> AQVINTFDGVADYLQTYHKLPDNYITKSEAQALGWVASKGNLADVAPGKSIGGDIFSNREGKLP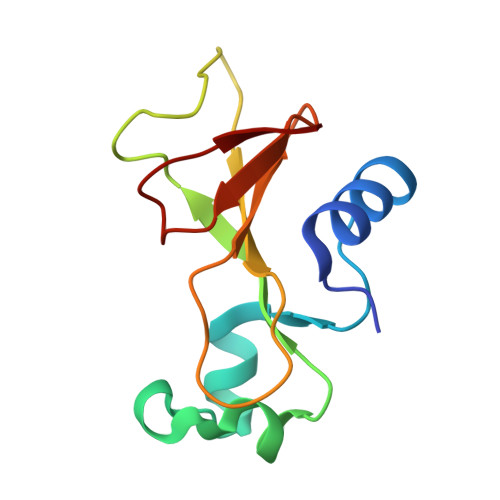GKSGRTWREADINYTSGFRNSDRILYSSDWLIYATTDHYQTFTKIR4-[(5-bromanylisoquinolin-3-yl)amino]-4-oxidanylidene-butanoic acid | C13 H11 Br N2 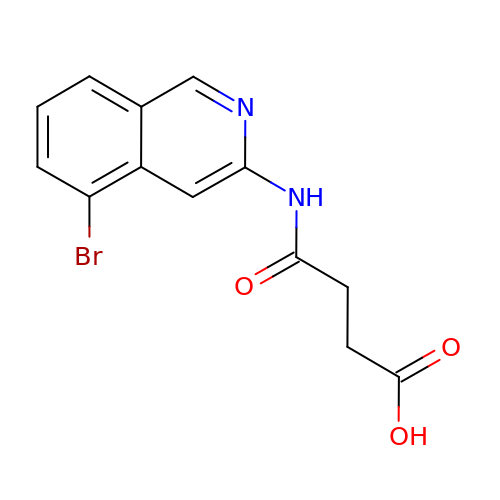O3 | AJBZFYAXPKNJJI-UHFFFAOYSA-N>VDQVGVTDFTADKTSAKADGTEAITYTATVKKNGVAQANVPVSFNIVSGTAVLSANSANTNGSGKATVTLKSDKPGQVVVSAKTAEMTSALNANAVIFVDQTKASITEIKADKTTAVANGQDAITYTVKVMKGDKPVSNQEVTFTTTLGKLSNSTEKTDTNGYAKVTLTSTTPGKSLVSARVSDVAVDVKAPEVEFFTT[2x]

Intimin is a 94 kDa outer membrane protein, essential for the intimate attachment of bacterial cells to the host cell surface, followed by actin pedestal formation. Intimin is classified as an inverse autotransporter, a subclass of the type 5 secretion system that transports the C-terminal extracellular region or passenger through the lumen of the N-terminal β-barrel located in the outer membrane. The intimin passenger forms a rod-like extension consisting of four tandem bacterial immunoglobulin-like (Big) domains (subdomains D00–D0–D1–D2) capped by a C-terminal C-type lectin-like domain (D3). Here, we describe the crystal structures of the combined intimin domains D00–D0 and D0–D1 from the EPEC strain E2348/69 determined at 1.5 Å and 1.8 Å resolution, respectively.

By contrast, the crystal structure of D0–D1 exhibits a kink between the two subdomains, leading to an approximately 45° angle between the two and a distance between the N- and C-termini of only 36 Å. Here, we show that D0 and D1 exhibit a seven-stranded strand-switched type (s-type) fold. Additionally, intimin D0 is structurally highly similar to D1 with a root mean square deviation (RMSD) of 0.68 Å and 0.84 Å with invasin subdomain D1 while sharing little structural conservation with the intimin subdomain D00 (RMSD: 4.68 Å). EOM analysis of D0–D1 revealed the presence of two conformational states, a bent and an elongated conformation. The bent conformation fits the kinked crystal structure of D0–D1. The equilibrium is shifted towards the bent form in comparison to the extended one with a volume fraction of 0.8:0.2. Based on this definition, the crystal structures of D00–D0 and D0–D1 have θ ~ 170° and θ ~ 60°, respectively. Figure 4a shows that D00–D0 adopts extended conformations characterized by a narrow, approximately bell-shaped distribution of θ centered around 140° whereas D0–D1 is considerably more flexible and explores a wider range of domain-domain angles, including the strongly bent conformations. D1 is the most rigid domain and, interestingly, D0 is considerably more flexible in D0–D1 than in D00–D0. The best crystals of D0–D1 were obtained in 0.1 M tris, pH 8.5; 0.2 M magnesium chloride hexahydrate and 25% polyethylene glycol 3350 (PEG3350). The flexibility demonstrated by the D0–D1 and D1–D2 connectors is also likely to be functionally important.>[2x]MAAGESMAQRMVWVDLEMTGLDIEKDQIIEMACLITDSDLNILAEGPNLIIKQPDELLDSMSDWCKEHHGKSGLTKAVKESTIT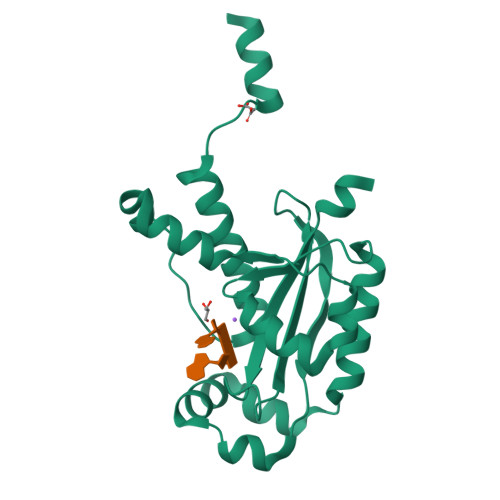LQQAEYEFLSFVRQQTPPGLCPLAGNSVHEDKKFLDKYMPQFMKHLHYRIIDVSTVKELCRRWYPEEYEFAPKKAASHRALDDISESIKELQFYRNNIFKKKIDEKKRKIIENGENEKTVS> MELKHSISD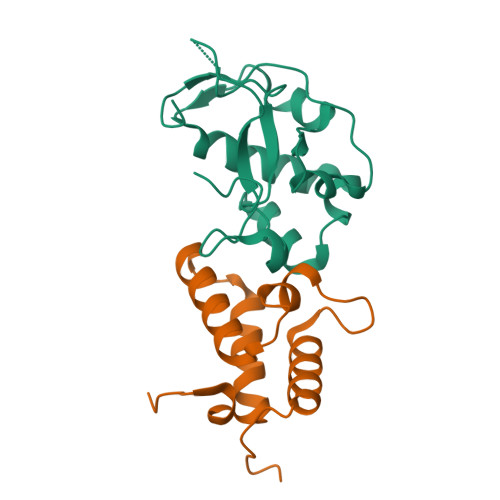YTEAEFLEFVKKIEDANSSEDEQQKLVEEFIRLTEHPSGSDLIYYPRDDREDSPEGIVKEIKEWRAANGKSGFKQGLEHHHHHH;> MESKRNKPGKATGKGKPVGDKWLDDAGKDSGAPIPDRIADKLRDKEFKNFDDFRKKFWEEVSKDPDLAKQFKRSNRKRIQQGYAPFAPQKDQVGGRTTFELHHDKPISQDGGVYDMNNIRVTTPKRAIDIHRGK>GAMGSKLSYTSFVQMVE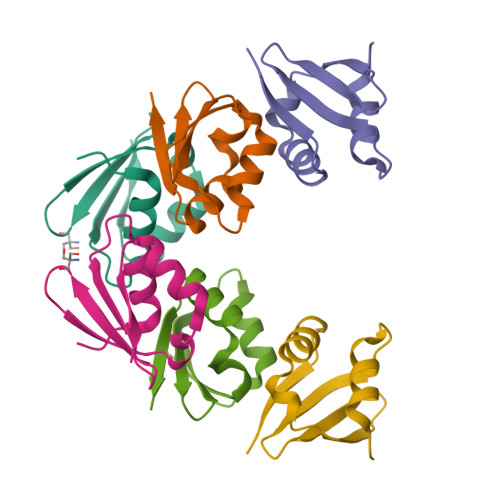DERSVVSEVVIRDDGVLRVYTKDGRVYEVDAPWAVNDSQLIEKLVSKGIKVSGER[3x]> MNSIIQRISKFDNILKDKTIINQQDLRQISWNGIPKIHRPVVWKLLIGYLPVNTKRQEGFLQRKRKEYRDSLKHTFSDQHSRDIPTWHQIEIDIPRTNPHIPLYQFKSVQNSLQRILYLWAIRHPASGYVQGINDLVTPFFETFLTEYLPPSQIDDVEIKDPS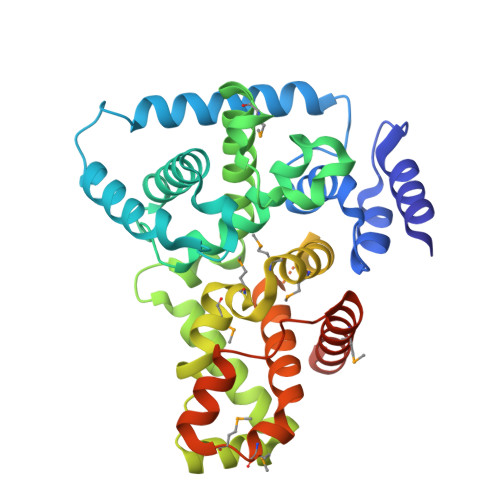TYMVDEQITDLEADTFWCLTKLLEQITDNYIHGQPGILRQVKNLSQLVKRIDADLYNHFQNEHVEFIQFAFRWMNCLLMREFQMGTVIRMWDTYLSETSQEVTSSYSMSSNDIKPPVTPTEPRVASFVTPTKDFQSPTTALSNMTPNNAVEDSGKMRQSSLNEFHVFVCAAFLIKWSDQLMEMDFQETITFLQNPPTKDWTETDIEMLLSEAFIWQSLYKDATSHWLHHHHHH diethyl 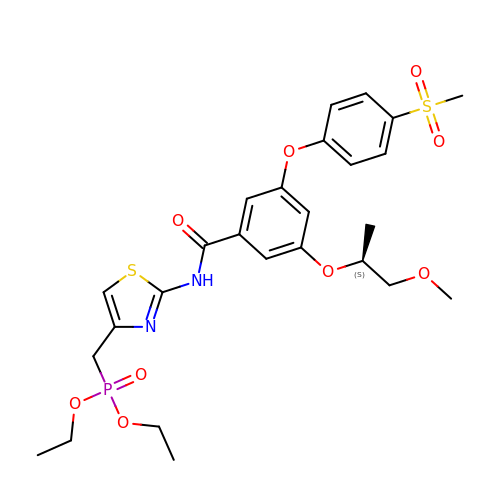{[2-(3-[4-(methanesulfonyl)phenoxy]-5-{[(2S)-1-methoxypropan-2-yl]oxy}benzamido)-1,3-thiazol-4-yl]methyl}phosphonate | C26 H33 N2 O9 P S2 | OQUMCVQSAWPKMT-SFHVURJKSA-N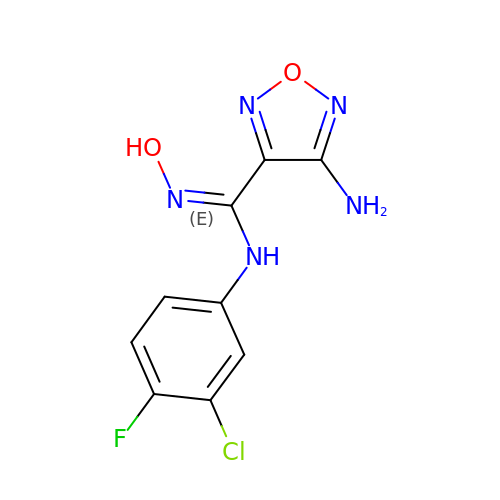4-Amino-N-(3-chloro-4-fluorophenyl)-N'-hydroxy-1,2,5-oxadiazole-3-carboxamidine | C9 H7 Cl F N5 O2 | HGXSLPIXNPASGZ-UHFFFAOYSA-N The mitochondrial calcium uniporter (MCU) is responsible for mitochondrial calcium uptake and homeostasis. MCU consists of two conserved transmembrane helices (TMs) connected by a 9‐aa linker with a four‐residue “DIME” motif flanked by an N‐terminal domain (NTD) and C‐terminal domain located within the mitochondrial matrix 11, 12, 13. MCU is associated with many regulatory proteins such as mitochondrial calcium uptake‐1 and mitochondrial calcium uptake‐2 (MICU1 and MICU2), an MCU paralog (MCUb), and essential MCU regulator (EMRE), forming the mitochondrial calcium uniporter complex (uniplex) 3, 4, 5, 6, 7. MCU NTD appears to be essential for the regulation of mitochondrial Ca2+ uptake through interaction with regulator(s) and/or modulation of post‐translational modifications.

The T4 lysozyme fusion was used to enhance solubility and to phase a new crystal structure using molecular replacement. We also determined the structure of an extended version of the MCU NTD (MCU NTD‐E), corresponding to residues 75–185, without the T4 lysozyme fusion at a 1.50 Å resolution (Figs 1 and EV1B). The structure of MCU NTD‐E was determined by molecular replacement using the MCU NTD structure as a template. Superposition of the two structures revealed a root mean square deviation (RMSD) of 0.29 Å for 90 Cα atoms. MCU NTD‐E has an additional α‐helix (α3) and a C‐terminal tail. In the structure of MCU NTD‐E, hydrophobic residues in the α2‐helix (L143, L144 and L146) together with L167 and L168 in the α3‐helix (166DLLSHENA173) form a hydrophobic surface surrounded by hydrophilic residues (namely D142, D166 and E171). This surface and C‐terminus tail (174ATLNNVKTL182) were predicted as potential protein–protein interaction (PPI) interfaces by the InterProSurf analysis 32 (Fig EV2A and C) and the consensus Protein–Protein Interaction Site Predictor (cons‐PPISP) server 33 (Fig EV2B and C). The C‐terminal tail in MCU NTD‐E forms an extended coil structure and contains K180, a known ubiquitination and biotinylation site 25, 26. Of interest, we observed an unidentified electron density, which is predicted as a linear lipid‐like molecule with 13–16 carbon atoms and modelled with a tetraethylene glycol molecule. The lipid‐like molecule interacts with the residues in the L1 loop, two helices (α2 and α3) and C‐terminus tail. In the crystal of MCU NTD‐E, oligomers are stabilized by additional interactions through an extended C‐terminal tail in a manner resembling domain swapping (Fig EV3B–D), and the interface in MCU NTD and the C‐terminal tail between subunits in the oligomer is consistent with the predicted PPI surface (Fig EV3E).

> MNHKVHHHHHHMVTVVYQNGLPVISVRLPSRRERCQFTLKPISDSVGVFLRQLQEEDRGIDRVAIYSPDGVRVAASTGIDLLLLDDFKLVINDLTYHVRPPKRDLLSHENAATLNDVKTLVQQ> IPEYVDWRQKGAVTPVKNQGSCGSCWAFSAVVTIEGIIKIRTGNLNQYSEQELLDCDRRSYGCNGGYPWSALQLVAQYGIHYRNTYPYEGVQRYCRSREKGPYAAKTDGVRQVQPYNQGALLYSIANQPVSVVLQAAGKDFQLYRGGIFVGPCGNKVDHAVAAVGYGPNYILIKNSWGTGWGENGYIRIKRGTGNSY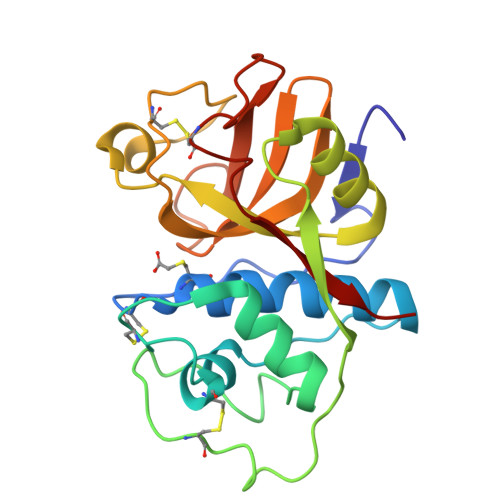GVCGLYTSSFYPVKN A novel cytoplasmic dye-decolorizing peroxidase from Dictyostelium discoideum was investigated that oxidizes anthraquinone dyes, lignin model compounds, and general peroxidase substrates such as ABTS efficiently. Dictyostelium DyPA is a dimer, with each monomer exhibiting a two-domain, α/β ferredoxin-like fold. In solution, Dictyostelium DyPA exists as a stable dimer with the side chain of Asp146 contributing to the stabilization of the dimer interface by extending the hydrogen bond network connecting two monomers. The active site of Dictyostelium DyPA has a hexa-coordinated heme iron with a histidine residue at the proximal axial position and either an activated oxygen or CN− molecule at the distal axial position.

Since earlier studies have shown that peroxidase–CN− complexes are a good and stable mimic of the peroxidase-H2O2 bound state, we recorded the UV-Vis spectra of Dictyostelium DyPA at pH 8.0 in the presence of KCN. The absorption spectrum suggests that the binding of CN− leads to a change in the electronic state of iron from high spin to low spin. To understand the binding mode of H2O2, we crystallized and solved the structure of Dictyostelium DyPA-CN− to 1.85 Å. The asymmetric unit contains two copies of the complex. Though the binding mode of H2O2 and cyanide differ, the position of the carbon atom still mimics the position of the iron-coordinated oxygen of H2O2 during the formation of compound I. Therefore, the position of the cyanide can provide information about possible interactions between Asp149 and the iron-coordinated oxygen of H2O2. Superposition of the Dictyostelium DyPA:O2 and the cyanide complex structures shows a minor change in Cα-RMSD of 0.13 Å. The cyanide molecule takes the place of the O2 molecule in the DyPA:O2 complex structure. No changes in the conformation of active site residues are observed. This is different from the situation reported for the BadDyP-CN− complex, where a change in the location of the aspartate side chain was reported. Our O2 complex structure, as well as the CN− complex structure, shows the Asp149 in hydrogen bonding distance to the proximal oxygen of H2O2, suggesting that Asp149 can accept a proton from H2O2 and compound I can form without side-chain movement.

>GPLGSMAQSTVLPMHCLYGIFLEGNLKIQKNDQEGLKKFKDNIKKFTLELDEIDKISPQSRIGGAICFSSDIWDTVTKKISKPKELKSVNTLSSYMPGTSQRDILIHIISDRMDTCFKLAQDTMRNFGEDQLDIKQEIHGFRRVEERDLTDFIDGTENPDGDELRTQYGLVAAGQPNEFGSYVFTQRYVHNLKKWYPEPLSVQQDTVGRTKKDSIEIPRDKRPITSHVSRTDLSENGKDLKIVRQSLPYGQITGEKGLMFIAYACSLHNIEKQLQSMFGQLDGKHDLLLKYTTPVTGSFYFAPSKKELLEL[2x]>DSVLLSGQTLYAGHSLTSGSYTLTIQNNCNLVKYQHGRQIWASDTDGQGSQCRLTLRSDGNLIIYDDNNMVVWGSDCWGNNGTYALVLQQDGLFVIYGPVLWPLGLNGCRSLN[4x];>DNVLLSGQTLHADHSLQA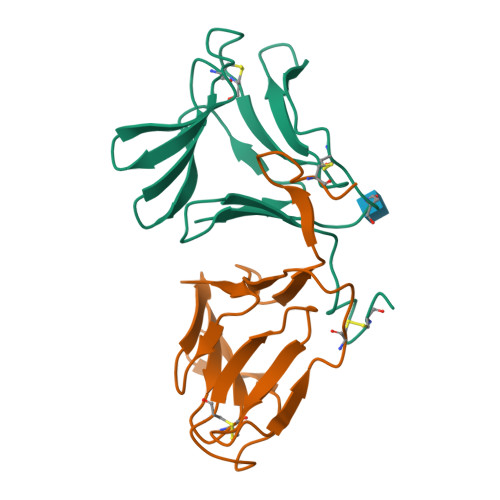GAYTLTIQNKCNLVKYQNGRQIWASNTDRRGSGCRLTLLSDGNLVIYDHNNNDVWGSACWGDNGKYALVLQKDGRFVIYGPVLWSLGPNGCRRVNG[4x]>[36x]XGEIAQGLKEIAKGLKE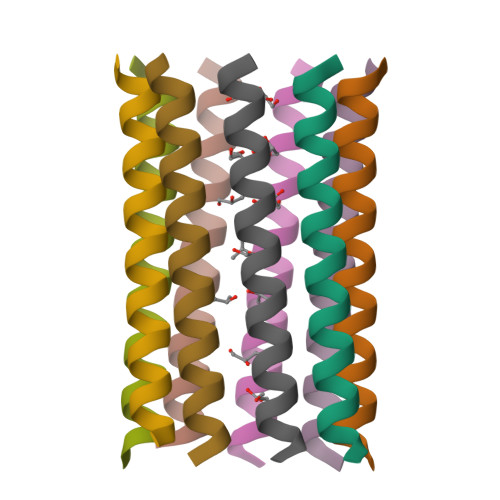IAWGLKEIAQGLKGX>[2x]MDEFEMIKRNTSEIISEEELREVLKKDEKSALIGFEPSGKIHLGHYLQI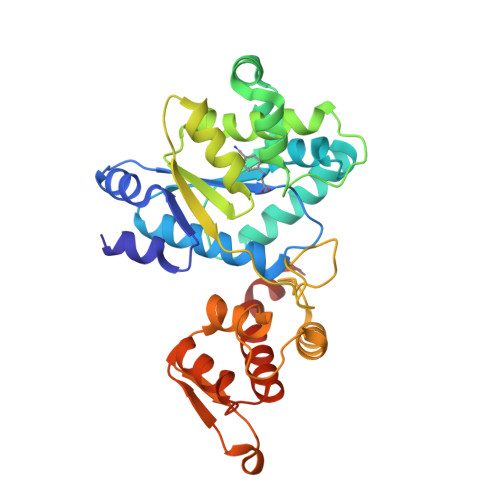KKMIDLQNAGFDIIIVLADLHAYLNQKGELDEIRKIGDYNKKVFEAMGLKAKYVYGSEWMLDKDYTLNVYRLALKTTLKRARRSMELIAREDENPKVAEVIYPIMQVNGAHYLGVDVAVGGMEQRKIHMLARELLPKKVVCIHNPVLTGLDGEGKMSSSKGNFIAVDDSPEEIRAKIKKAYCPAGVVEGNPIMEIAKYFLEYPLTIKRPEKFGGDLTVNSYEELESLFKNKELHPMDLKNAVAEELIKILEPIRKRLLIRKRL10,11-dimethoxy-4-methyldibenzo[c,f]-2,7-naphthyridine-3,6-diamine | 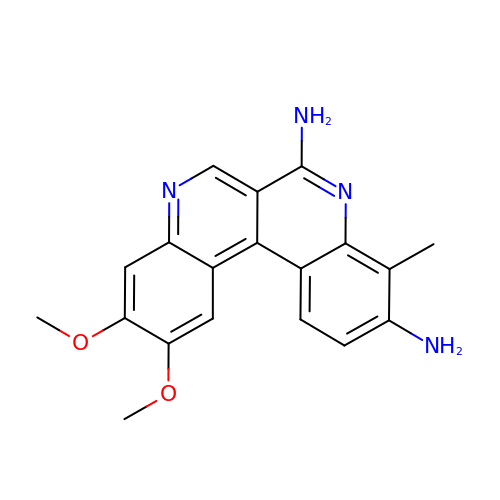C19 H18 N4 O2 | NVINUNQBDNEMSY-UHFFFAOYSA-N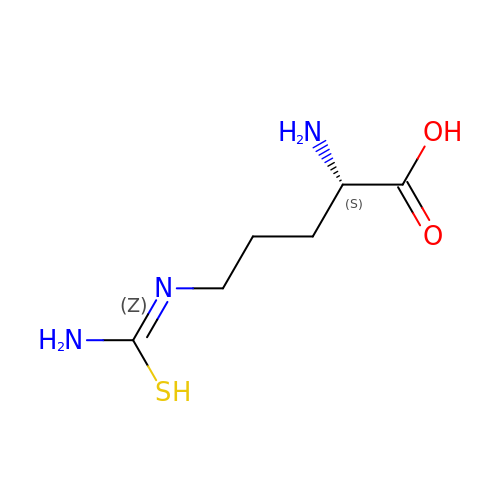L-THIOCITRULLINE | C6 H13 N3 O2 S | BKGWACHYAMTLAF-BYPYZUCNSA-N>MSPQAQGLGVDGACRPCSDAELLLAACTSDFVIHGTIHGVAHDTELQESVITVVVARVIRQTLPLFKEGSSEGQGRASIRTLLRCGVRPGPGSFLFMGWSRFGEAWLGCAPRFQEFSRVYSAALTTHL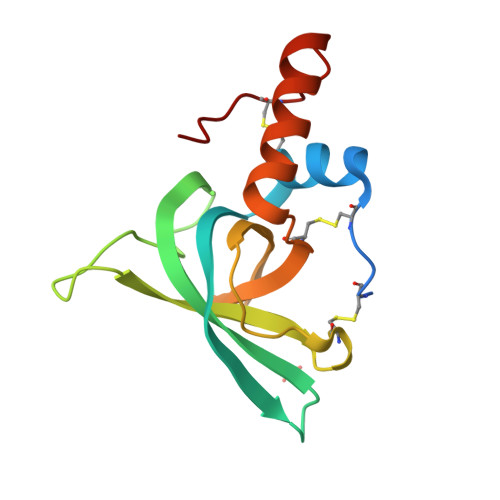NPCEMALD[4x]> NLYQFKNMIQCTVPSRSWADFADYGCYCGKGGSGTPVDDLDRCCQTHDNCYNEAENISGCRPYFKTYSYECTQGTLTCKGDNNACAASVCDCDRLAAICFAGAPYNDDNYNIDLKARCN;> LA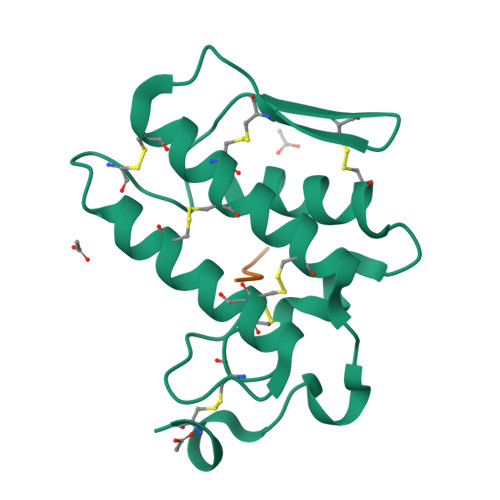IYS>MTTAAGLSGIDLTDLDNFADGFPHHLFAIHRREAPVYWHRPTEHTPDGEGFWSVATYAETLEVLRDPVTYSSVTGGQRRFGGTVLQDLPVAGQVLNMMDDPRHTRIRRLVSSGLTPRMIRRVEDDLRRRARGLLDGVEPGAPFDFVVEIAAELPMQMICILLGVPETDRHWLFEAVEPGFDFRGSRRATMPRLNVEDAGSRLYTYALELIAGKRAEPADDMLSVVANATIDDPDAPALSDAELYLFFHLLFSAGAETTRNSIAGGLLALAENPDQLQTLRSDFELLPTAIEEIVRWTSPSPSKRRTASRAVSLGGQPIEAGQKVVVWEGSANRDPSVFDRADEFDITRKPNPHLGFGQGVHYCLGANLARLELRVLFEELLSRFGSVRVVEPAEWTRSNRHTGIRHLVVELRGG[2x]

Among these is CYP126A1, a P450 with ∼35% amino acid identity to the cholesterol-oxidizing M. tuberculosis CYP142A1 and CYP125A1. However, CYP126A1 is highly conserved across pathogenic and non-pathogenic Mycobacterium species, suggesting an important evolutionary role for the protein. In conclusion, we present the first biochemical and structural studies of the M. tuberculosis P450 CYP126A1, revealing novel substrates and inhibitors for the enzyme, defining its relatively polar active site and its ability to adapt structurally to facilitate the binding of bulky ligands. The CYP126A1 structures reveal a dynamic molecule, with the BC and FG regions clearly affected by ligand binding.

Unlike the previous ligands, compound 1 does not contain an azole ring and instead elicits a type I heme shift suggestive of substrate-like ligand binding. The crystal structure of CYP126A1 in complex with compound 1 reveals that the ligand is bound with the nitrobenzene moiety placed directly above and parallel to the heme porphyrin plane. This effectively ensures that the heme iron sixth ligand water is displaced, explaining the observed spectroscopic effect with HS heme iron formation. As observed for the azole-containing ligands, the binding of compound 1 elicits a shift in the N-terminal region of the I-helix to accommodate the nitrobenzene moiety, accompanied by the reorientation of the FG-helix region. As observed for compound 7, the BC-loop region appears unperturbed by compound 1 binding. However, the putative dimer interface observed in the CYP126A1-compound 1 complex is distinct in nature. Although still composed of interactions between the FG- and BC-loop regions, the respective orientation of both monomers is altered. Thus, binding of compound 1 results in a 155-mV increase in the CYP126A1 midpoint potential, consistent with heme iron reduction being favored in a substrate-bound form of the P450 (42). No evidence of oxidation of either compound 1 or compound 2 (which both possess a terminal 4-nitrophenyl group) could be obtained in turnover studies, and it thus appears that these molecules “moonlight” as substrates but are not readily oxidized and instead act as P450 inhibitors. However, two of the HTS molecules (compounds 1 and 3) were calculated to bind twice per CYP126A1 monomer at 5:1 ligand/protein ratios.> GPGSMKEQLLYLSKLLDFEVNFSDYPKGNHNEFLTIVTLSTHPPQICHGVGKSSEESQ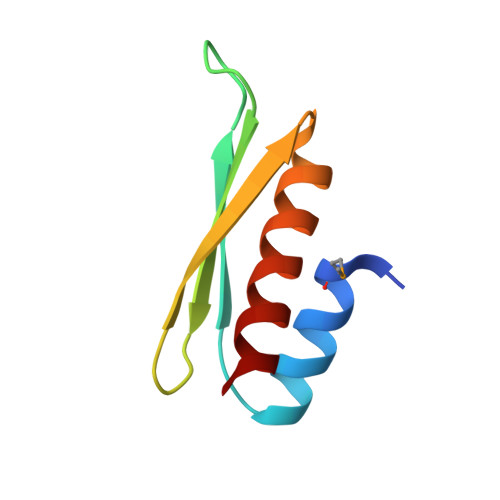NDAASNALKILSKL> MSETRMAQNMDTTDEQYLRLIELLSNYDSTLEQLQKGFQDGYIQLSRSNYYNKDSLRGNYGEDYWDETYIGQLMATVEEKNSKVVVEIVKRKAQDKQEKKEEEDNKLTQRKKGTKPEKQKTQSHKLKQDYDPILMFGGVLSVPSSLRQSQTSFKGCIPLIAQLINYKNEILTLVETLSEQE;> MFEIKLNDRITEFLRKFKNSAKSNEGIDEDIDLFLKRHAIPMQSLLFYVKEYRKDSDLQCSIKELLKPLEFEFKPKAVRGLHYSEDFKKKLEFLKYQEQELEYQSMVKRSKSVFSLQEDDELTPSQINKQIKEQVTTVFNVLVSVISVVVAIWYWTGSSTNFPVHVRLLLCLFFGILVLVADVVVYNSYLKKLEEAKVKEKTKVEKKKVLSKITL;> MAEKRTLIAVIADEDTTTGLLLAGIGQITPETQEKNFFVYQEGKTTKEEITDKFNHFTEERDDIAILLINQHIAENIRARVDSFTNAFPAILEIPSKDHPYDPEKDSVLKRVRKLFGE;> MVFGQLYALFIFTLSCCISKTVQADSSKESSSFISFDKESNWDTISTISSTADVISSVDSAIAVFEFDNFSLLDNLMIDEEYPFFNRFFANDVSLTVHDDSPLNISQSLSPIMEQFTVDELPESASDLLYEYSLDDKSIVLFKFTSDAYDLKKLDEFIDSCLSFLEDKSGDNLTVVINSLGWAFEDEDGDDEYATEETLSHHDNNKGKEGDDDILSSIWTEGLLMCLIVSALLLFILIVALSWISNLDITYGAL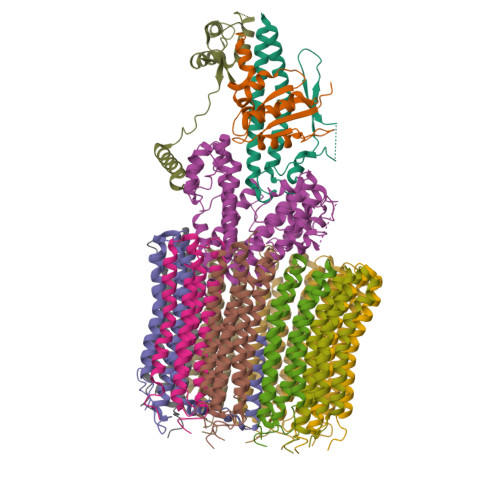EKSTNPIKKNN;> MNKESKDDDMSLGKFSFSHFLYYLVLIVVIVYGLYKLFTGHGSDINFGKFLLRTSPYMWANLGIALCVGLSVVGAAWGIFITGSSMIGAGVRAPRITTKNLISIIFCEVVAIYGLIIAIVFSSKLTVATAENMYSKSNLYTGYSLFWAGITVGASNLICGIAVGITGATAAISDAADSALFVKILVIEIFGSILGLLGLIVGLLMAGKASEFQ;> MEGVYFNIDNGFIEGVVRGYRNGLLSNNQYINLTQCDTLEDLKLQLSSTDYGNFLSSVSSESLTTSLIQEYASSKLYHEFNYIRDQSSGSTRKFMDYITYGYMIDNVALMITGTIHDRDKGEILQRCHPLGWFDTLPTLSVATDLESLYETVLVDTPLAPYFKNCFDTAEELDDMNIEIIRNKLYKAYLEDFYNFVTEEIPEPAKECMQTLLGFEADRRSINIALNSLQSSDIDPDLKSDLLPNIGKLYPLATFHLAQAQDFEGVRAALANVYEYRGFLETGNLEDHFYQLEMELCRDAFTQQFAISTVWAWMKSKEQEVRNITWIAECIAQNQRERINNYISVY;>[8x]MTELCPVYAPFFGAIGCASAIIFTSLGAAYGTAKSGVGICATCVLRPDLLFKNIVPVIMAGIIAIYGLVVSVLVCYSLGQKQALYTGFIQLGAGLSVGLSGLAAGFAIGIVGDAGVRGSSQQPRLFVGMILILIFAEVLGLYGLIVALLLNSRATQDVVC;> MSTQLASNIYAPLYAPFFGFAGCAAAMVLSCLGAAIGTAKSGIGIAGIGTFKPELIMKSLIPVVMSGILAIYGLVVAVLIAGNLSPTEDYTLFNGFMHLSCGLCVGFACLSSGYAIGMVGDVGVRKYMHQPRLFVGIVLILIFSEVLGLYGMIVALILNTRGSE>XAEIEQIKKEIAYLIKKIKEEILEE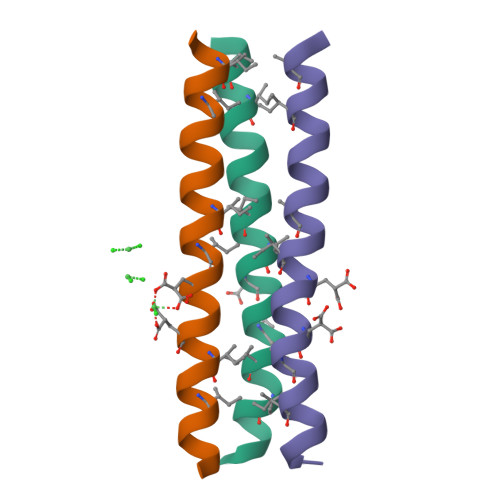IKKIKQEIA[3x]>GILELAGTVGCVGPRTPIAYMKYGCFCGLGGHGQPRDAIDWCCHGHDCCYTRAEEAGCSPKTERYSWQCVNQSVLCGPAEN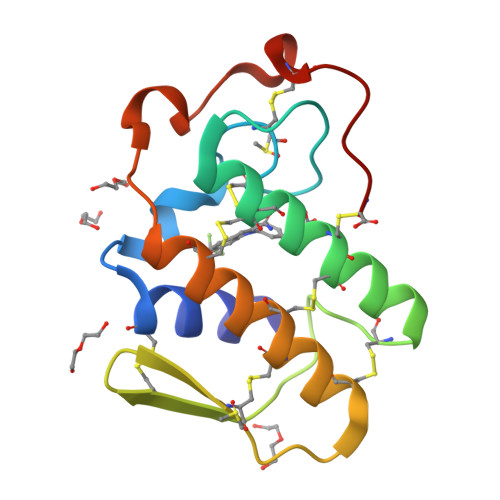KCQELLCKCDQEIANCLAQTEYNLKYLFYPQFLCEPDSPKC[2x]(3~{S})-3-[(4~{S})-3-aminocarbonyl-1-[(2~{R},3~{R},4~{S},5~{R})-5-[[[[(2~{R},3~{R},4~{R},5~{R})-5-(6-aminopurin-9-yl)-3-oxidanyl-4-phosphonooxy-oxolan-2-yl]methoxy-oxidanyl-phosphoryl]oxy-oxidanyl-phosphoryl]oxymethyl]-3,4-bis(oxidanyl)oxolan-2-yl]-4~{H}-pyridin-4-yl]-2-oxidanylidene-pentanedioic 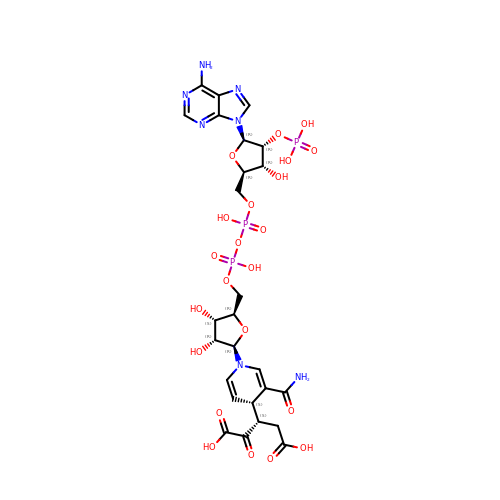acid | C26 H34 N7 O22 P3 | WSGZIHXYYXDDDT-PJNAXEGASA-N> MGSDKIHHHHHHMNIYDQLQAVEDRYEELGELLSDPDVVSDTKRFMELSREEANSRETVA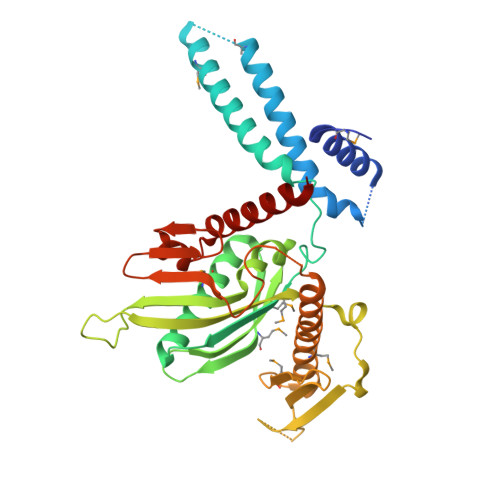VYREYKQVVQNIADAQEMIKDASGDPELEEMAKEELKNSKVAKEEYEEKLRFLLLPKDPNDDKNIILEIRGAAGGDEAALFAGDLLNMYQKYAENQGWKFEVMEASANGVGGLKEVVAMVSGQSVYSKLKYESGAHRVQRVPVTESQGRVHTSTATVLVMPEVEEVEYEIDPKDLRVDIYHASGAGGQNVNKVATAVRIIHLPTNIKVEMQEERTQQKNRDKAMKIIRARVADHFAQIAQDEQDAERKSTVGTGDRSERIRTYNFPQNRVTDHRIGLTLQKLDSILSGKLDEVIDALILYDQTQKLEELNK>[8x]GMPAQSPLRDGDTADFELIETMRWQPGTSFLRFDRHLARLYGSA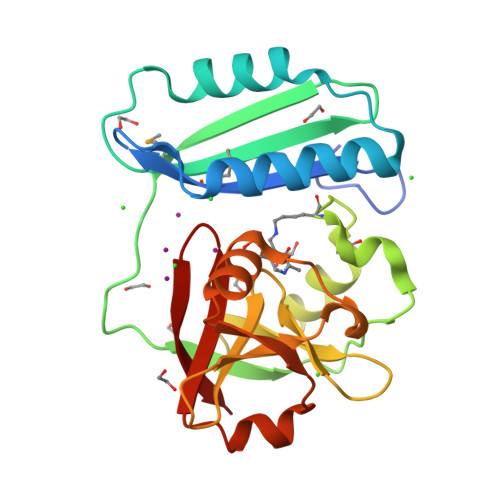AELGFACDPQRIAEVLSDALDGARTAMRTRLALARNGDATASAQPYEPLAADKVWILRLARTRLDSQNTLLRHKTSRRQLYTHARSEYLVTQADEVLLANERGEICEGTITNVFADFGDGVLATPRLDCGLLPGVLRAELLDEGRAEEAIYSYDDLKSAKALFVGNSLRGLIPAKLV>[2x]MERGEIWLVSLDPTAGHEQQGTRPVLIVTPAAFNRVTRLPVVVPVTSGGNFARTAGF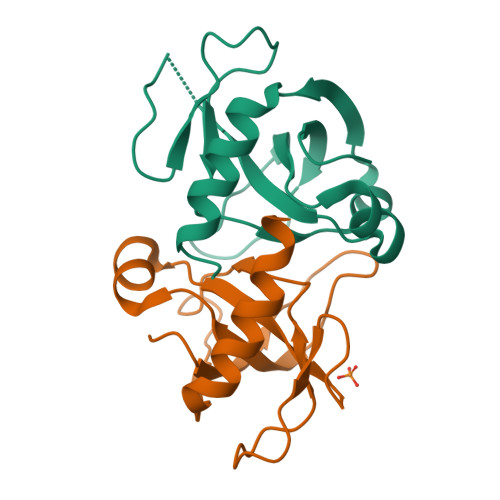AVSLDGVGIRTTGVVRCDQPRTIDMKARGGKRLERVPETIMNEVLGRLSTILT>MSLKENK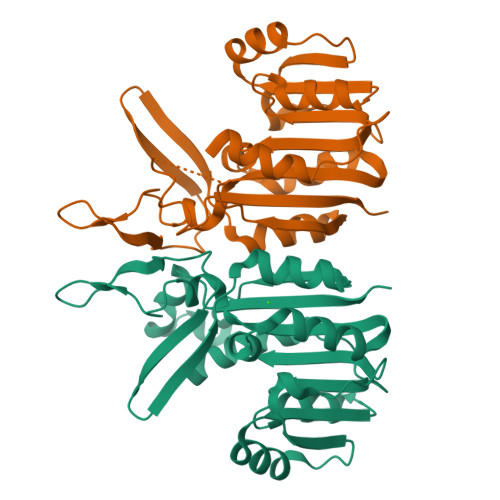YDDKHFFEQYSQMPRSKEGLKAAGEWHELKKMLPDFNQKTVLDLGCGFGWHCIYAAEHGAKKVLGIDLSERMLTEAKRKTTSPVVCYEQKAIEDIAIEPDAYNVVLSSLALHYIASFDDICKKVYINLKSSGSFIFSVEHPVFTADGRQDWYTDETGNKLHWPVDRYFNESMRTSHFLGEDVQKYHRTVTTYIQTLLKNGFQINSVIEPEPAPELKDLPEMQDEYRRPMMLLISATKQEGHHHHHH[2x]>[12x]MAIIETTTPTEEEAKAIAKKLLENRLIAEAIITPALTKIYRENGEIKSETVTRVTLYTEEEN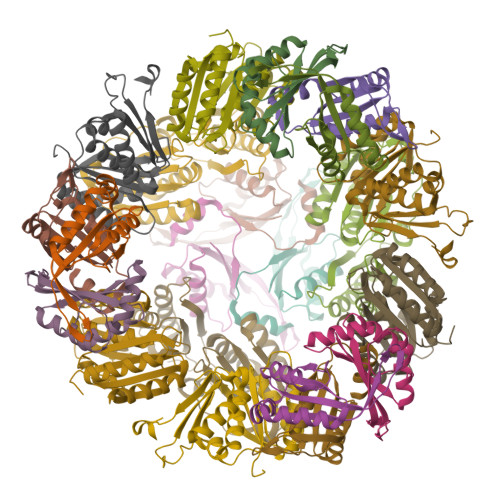VPKAVTYIKAIHPDPIPPIIVITPTDANPAYKGWVAFET;>DPERPALGILELSSYARGVKVADAALKAAPVKLLKCEPVEPGRALIMLLGEPEDVAKAMIAALDVAGLGSGNLIDYALIPEIHPQLLPFLKEYKKSEPIKDPNKAIIVAEVSTVAAAIEAADVALRLANVELTSMRLAEHIGGRASFTLIGDKEDVEKAARAIRGVAGERLLDLEIIEKPVEALIGNEFF[9x]> MASIKKVYRGMKNGAETINDDLEAINSELTSGGNVVHK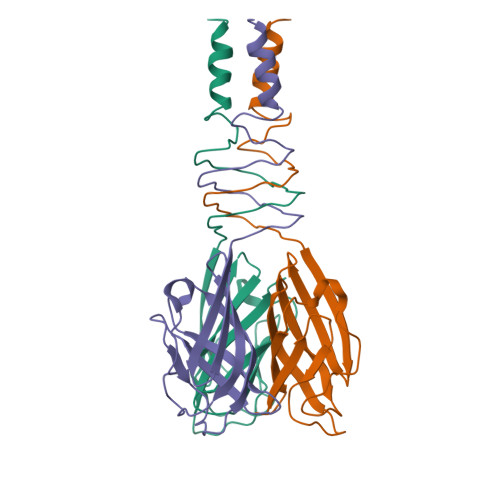TGDETIAGKKTFTGNVEVNGSLTLPVQTLTVEAGNGLQLQLTKKNNDLVIVRFFGSVSNIQKGWNMSGTWVDRPFRPAAVQSLVGHFAGRDTSFHIDINPNGSITWWGANIDKTPIATRGNGSYFIK>HHHHHHGCMSGRKPIIGVMGPGKADTAENQLVMANELGKQIATHGWILLTGGRSLGVMHEAMKGAKEAGGTTIGVLPGPDTSEISDAVDIPIVTGLGSARDNINALSSNVLVAVGMGPGTAAEVALALKAK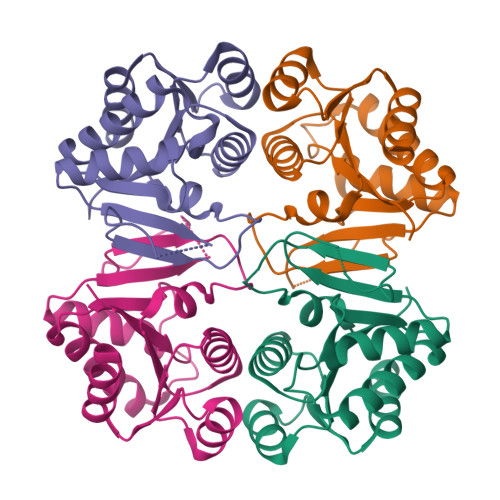KPVVLLGTQPEAEKFFTSLDAGLVHVAADVAGAIAAVKQLLAKLN[4x]> MADVTGIALGMIETRGLVPAIEAADAMTKAAEVRLVGRQFVGGGYVTVLVRGETGAVNAAVRAGADACERVGDGLVAAHIIARVHSEVENILPKAPQA

The prototypical bacterial microcompartment is the carboxysome, which is found in many bacteria that fix CO2 into organic carbon. The carboxysome shell is formed mainly by the assembly of many copies of a few small shell proteins. Here the crystal structure is reported for CsoS1A. This protein and the nearly identical CsoS1C protein are the main constituents of the alpha carboxysome shell in the chemoautotroph H. neapolitanus. CsoS1A forms a cyclic hexameric building block from six monomeric subunits, as observed previously in the CcmK2 and CcmK4 shell subunits from Syn.

However, it was possible to visualize bound sulfate ions after soaking a crystal in 200 mM sodium sulfate. Sulfate can be considered an analog for bicarbonate, having a similar size and a charge of the same sign, though twice as large in magnitude. Difference electron density maps suggested possible sulfate ions at three locations. One of these sites was in the hexagonal pore, whereas the others were at the locations where the 2-fold and 3-fold axes of symmetry pass through the layer, i.e., where two hexamers meet at an edge and where three meet at a corner. Sulfur atoms scatter X-rays anomalously, so an anomalous difference Fourier map was used to visualize possible sulfate ions. This calculation confirmed the sulfate ion in the hexagonal pore, but was not definitive with regard to the other putative sulfate binding sites. In the hexagonal pore, the sulfate is in contact with Gly43, which is part of a Gly-Gly-Gly motif that is conserved across the three CsoS1 proteins (A, B, and C) and other closely related shell proteins, but not in the CcmK proteins. The negatively charged sulfate oxygen atoms are poised to make hydrogen bonds to the backbone amide nitrogen of Gly43, and possibly to the C-alpha hydrogen atom of that residue; the potential importance of hydrogen bonds involving C-alpha hydrogen atoms has been discussed, but their strength remains an open question. The visualization of sulfate ions inside the pores of the CsoS1A layer indicates that transport of small molecules such as bicarbonate is probably feasible. Recall that sulfate (carrying a −2 charge) could be seen bound in the pore, whereas the natural intermediate bicarbonate was not seen to be tightly bound.> MAGDKGGGDGERRLRQPIVVVLGHVDHGKTTLLDKIRRTAVAAKEAGGITQHIGASIVPADVIEKIAEPLKKVIPVKLVIPGLLFIDTPGHELFSNLRRRGGSVA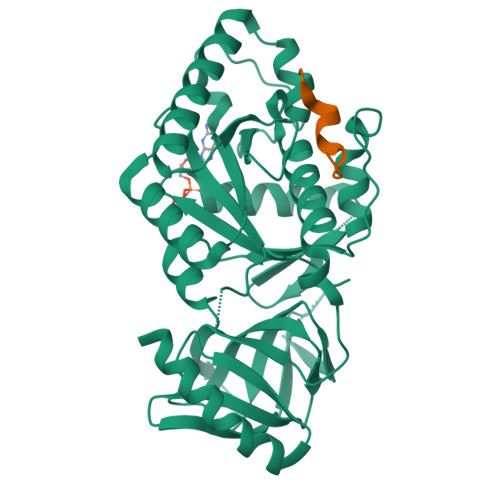DFAILVVDIMEGFKPQTYEALELLKERRVPFLIAANKIDRIPGWKPNPDAPFIETIRRQDPKVREILEQRVYEIVGKMYEAGLPAELFTRIKDFRRKIAIVPVSARTGEGIPELLAVLAGLTQTYLKERLRYAEGPAKGVVLEVKEMQGFGTVVDAVIYDGVLKKEDIIVVGGREGPIVTRVRALLMPAPLQDIRSREARFVQVDRVYAAAGVRIAAPGLDDVIAGSPIYAAESEEEARKLMEAVQREIEELRHHHHHH;> KKKKKKEEEVDLSGLSGMFGF> H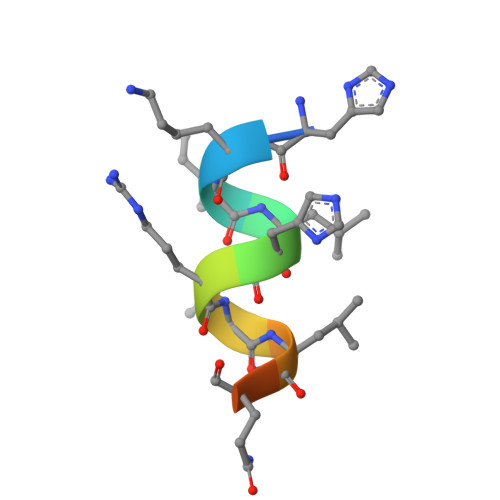KILHRLLQEGS>MERDGCAGGGSRGGEGGRAPREGPAGNGRDRGRSHAAEAPGDPQAAASLLAPMDVGEEPLEKAARARTAKDPNTYKVLSLVLSVCVLTTILGCIFGLKPSCAKEVKSCKGRCFERTFGNCRCDAACVELGNCCLDYQETCIEPEHIWTCNKFRCGEKRLTRSLCACSDDCKDKGDCCINYSSVCQGEKSWVEEPCESINEPQCPAGFETPPTLLFSLDGFRAEYLHTWGGLLPVISKLKKCGTYTKNMRPVYPTKTFPNHYSIVTGLYPESHGIIDNKMYDPKMNASFSLKSKEKFNPEWYKGEPIWVTAKYQGLKSGTFFWPGSDVEINGIFPDIYKMYNGSVPFEERILAVLQWLQLPKDERPHFYTLYLEEPDSSGHSYGPVSSEVIKALQRVDGMVGMLMDGLKELNLHRCLNLILISDHGMEQGSCKKYIYLNKYLGDVKNIKVIYGPAARLRPSDVPDKYYSFNYEGIARNLSCREPNQHFKPYLKHFLPKRLHFAKSDRIEPLTFYLDPQWQLALNPSERKYCGSGFHGSDNVFSNMQALFVGYGPGFKHGIEADTFENIEVYNLMCD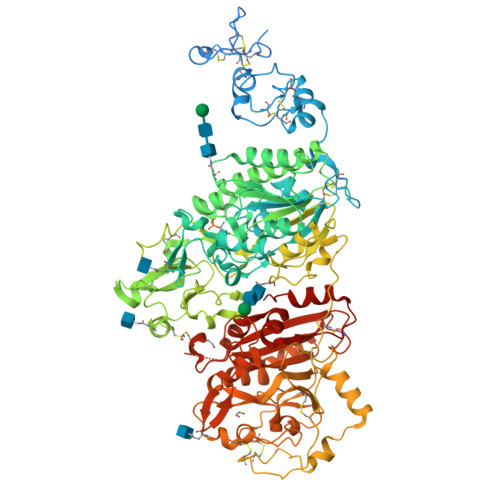LLNLTPAPNNGTHGSLNHLLKNPVYTPKHPKEVHPLVQCPFTRNPRDNLGCSCNPSILPIEDFQTQFNLTVAEEKIIKHETLPYGRPRVLQKENTICLLSQHQFMSGYSQDILMPLWTSYTVDRNDSFSTEDFSNCLYQDFRIPLSPVHKCSFYKNNTKVSYGFLSPPQLNKNSSGIYSEALLTTNIVPMYQSFQVIWRYFHDTLLRKYAEERNGVNVVSGPVFDFDYDGRCDSLENLRQKRRVIRNQEILIPTHFFIVLTSCKDTSQTPLHCENLDTLAFILPHRTDNSESCVHGKHDSSWVEELLMLHRARITDVEHITGLSFYQQRKEPVSDILKLKTHLPTFSQED[2x]>MKNVGFIGWRGMVGSVLMDRMSQENDFENLNPVFFTTSQAGQKAPVFGGKDAGDLKSAFDIEELKKLDIIVTCQGGDYTNEVYPKLKATGWDGYWVDAASALRMKDDAIIVLDPVNQHVISEGLKKGIKTFVGGNCTVSLMLMAIGGLFEKDLVEWISVATYQAASGAGAKNMRELLSQMGLLEQAVSSELKDPASSILDIERKVTAKMRADNFPTDNFGAALGGSLIPWIDKLLPETGQTKEEWKGYAETNKILGLSDNPIPVDGLCVRIGALRCHSQAFTIKLKKDLPLEEIEQIIASHNEWVKVIPNDKEITLRELTPAKVTGTLSVPVG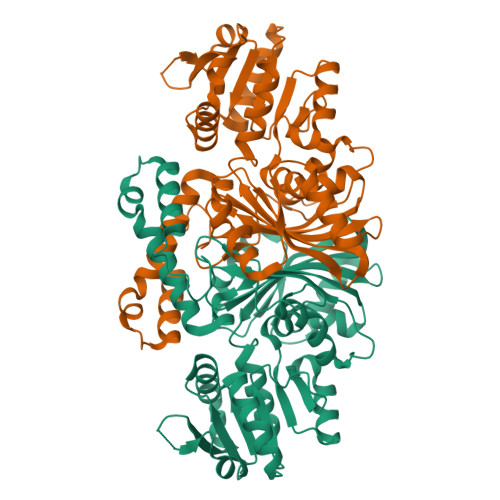RLRKLAMGPEYLAAFTVGDQLLWGAAEPVRRILKQLVA[2x]> GT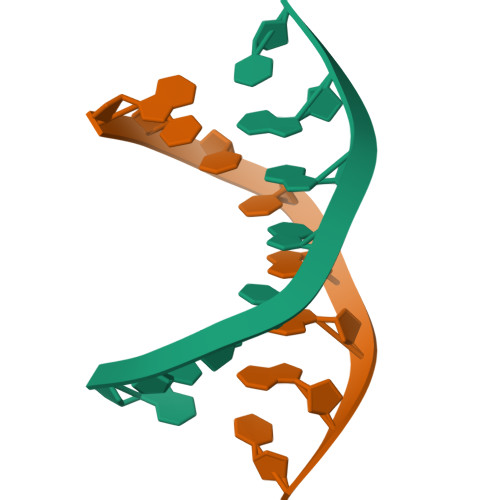CTAGAC> SPLAVGLAAHLRQIGGTMYGAYWCPHCQDQKELFGAAFDQVPYVECSPNGPGTPQAQECTEAGITSYPT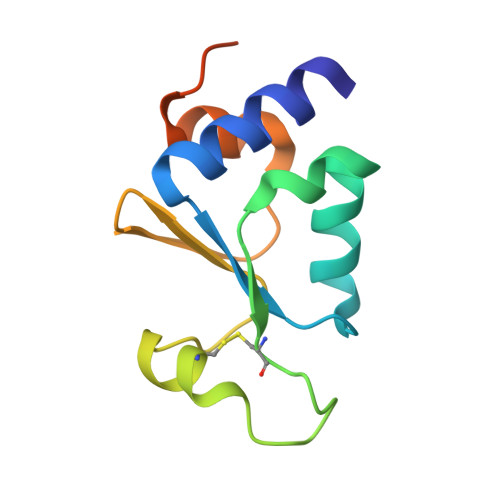WIINGRTYTGVRSLEALAVASGYPLEEGRLEHHHHHH Carboxysomes are specialized microcompartments found in all cyanobacteria and certain chemoautotrophic proteobacteria, playing a crucial role in CO2 fixation and serving as a central component of bacterial CO2-concentrating mechanisms. These organelles encapsulate 2 cargo enzymes: Ribulose-1,5-bisphosphate carboxylase/oxygenase (Rubisco) and carbonic anhydrase, using a polyhedral proteinaceous shell. Self-assembly of the α-carboxysome is mediated by the intrinsically disordered protein CsoS2. CsoS2 functions as a linker protein, connecting cargo enzymes like Rubisco with the shell proteins.

For instance, heterologous expression of minimal shell protein components derived from Halothiobacillus neapolitanus, including the hexameric shell protein CsoS1A, pentameric vertex CsoS4A, and CsoS2, allowed for the construction of a T = 9 icosahedral α-carboxysome shell with a maximum diameter of 36.9 nm. To address this issue, we reanalyzed our recently reported cryo-EM density maps without applying any symmetry (C1 symmetry). Fortunately, we were still able to obtain maps for the T = 9 and T = 16 α-carboxysome shells at resolutions of 2.77 Å and 3.71 Å, respectively. The construction of structures using C1 symmetry maps yielded T = 9 shells with a diameter of 36.9 nm and T = 16 shells with a diameter of 49.2 nm, which are virtually identical to the structures obtained under I symmetry. Nevertheless, in the T = 9 C1 symmetry map, no redundant density was detected, indicating that high-symmetry processing is unlikely to greatly impact the structural building in shells with smaller diameters. In summary, we show that excessive averaging in the highly symmetrical processing of α-carboxysome shell cryo-EM data can distort local densities, potentially leading to the loss of key structural details.

>MADVTGIALGMIETRGLVPAIEAADAMTKAAEVRLVGRQFVGGGYVTVLVRGETGAVNAAVRAGADACERVGDGLVAAHIIARVHSEVENILPKAPQA[480x];>MKIMQVEKTLVSTNRIADMGHKPLLVVWEKPGAPRQVAVDAIGCIPGDWVLCVGSSAAREAAGSKSYPSDLTIIGIIDQWNGE[60x];>MPSQSGMNPADLSGLSGKELARARRAALSKQGKAAVSNKTASVNRSTKQAASSINTNQVRSSVNEVPTDYQMADQLCSTIDHADFGTESNRVRDLCRQRREALSTIGKKAAKTTGKPSGRVRPQQSVVHNDAMIENAGDTNQSSSTSLNNELSEICSIADDMPERFGSQAKTVRDICRARRQALSERGTRAVPPKPQSQGGPGRNGYQIDGYLDTALHGRDAAKRHREMLCQYGRGTAPSCKPTGRVKNSVQSGNAAPKKVETGHTLSGGSVTGTQVDRKSHVTGNEPGTCRAVTGTEYVGTEQFTSFCNTSPKPNATKVNVTTTARGRPVSGTEVSRTEKVTGNESGVCRNVTGTEYMSNEAHFSLCGTAAKPSQADKVMFGATARTHQVVSGSDEFRPSSVTGNESGAKRTITGSQYADEGLARLTINGAPAKVARTHTFAGSDVTGTEIGRSTRVTGDESGSCRSISGTEYLSNEQFQSFCDTKPQRSPFKVGQDRTNKGQSVTGNLVDRSELVTGNEPGSCSRVTGSQYGQSKICGGGVGKVRSMRTLRGTSVSGQQLDHAPKMSGDERGGCMPVTGNEYYGREHFEPFCTSTPEPEAQSTEQSLTCEGQIISGTSVDASDLVTGNEIGEQQLISGDAYVGAQQTGCLPTSPRFNQTGNVQSMGFKNTNQPEQNFAPGEVMPTDFSIQTPARSAQNRITGNDIAPSGRITGPGMLATGLITGTPEFRHAARELVGSPQPMAMAMANRNKAAQAPVVQPEVVATQEKPELVCAPRSDQMDRVSGEGKERCHITGDDWSVNKHITGTAGQWASGRNPSMRGNARVVETSAFANRNVPKPEKPGSKITGSSGNDTQGSLITYSGGARG[60x]>[2x]QSGSGMRVGVLGAKG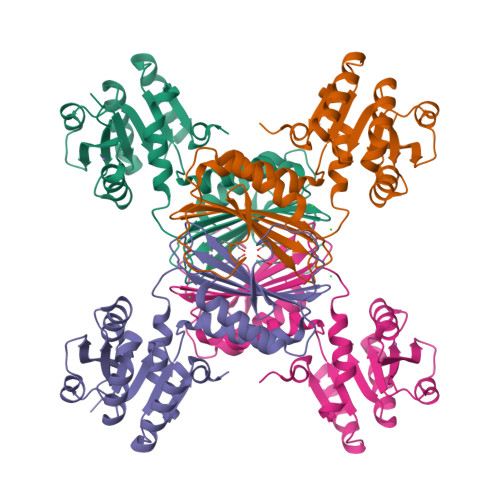KVGATMVRAVAAADDLTLSAELDAGDPLSLLTDGNTEVVIDFTHPDVVMGNLEFLIDNGIHAVVGTTGFTAERFQQVESWLVAKPNTSVLIAPNFAIGAVLSMHFAKQAARFFDSAEVIELHHPHKADAPSGTAARTAKLIAEARKGLPPNPDATSTSLPGARGADVDGIPVHAVRLAGLVAHQEVLFGTEGETLTIRHDSLDRTSFVPGVLLAVRRIAERPGLTVGLEPLLDLH> MLKRTLTVLDQTYGPHKSYKYTYMPDPRKLAPIETTQRSEIVPQSIRPPTSYVPNHETFLERADIHRLRPTSDFK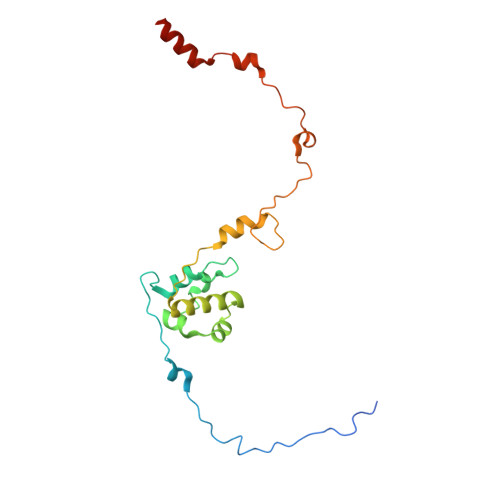ASFKDWNDLFTCDKRQLRVRGIPRMTRDAIRTAVQAFQNGNPPERFDTKEEWLYYKQFKTVDYSYRVIPELPEKYRPHQSGIDQAPLPDYREINKMPQWAECEERRQSKKTV> ELASSTSENSVETQEITTFHDVETPNRIDTPMAQDTSSARNMDDTHSIIQFLQRPVLIDNIEIIAG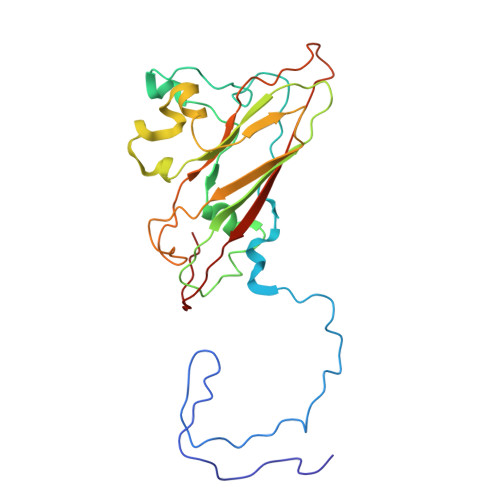TTADANKPLSRYVLDQQNSQKYVRSWTLPSTVLKAGGKAQKLANFKYLRCDVQVKLVLNANPFVAGRMYLAYSPYDDKVDTARSVLQTSRAGVTGYPGVELDFQLDNSVEMTIPYASFQEAYDLVTGTEDFVQLYLFPITPVLGPKSESESSKVDISVYMWLSNISLVIPTYRMNPD>GMFLLQGAQMLQMLEKSLRKSLPMSLKVYGTVMHMNHGNPFNLKALVDKWPDFQTVVIRPQEQDMKDDLDHYTNTYHVYSEDLKNCQEFLDLPEVINWKQHLQIQSTQSSLNEVIQNLAATKSFKVKRSKNILYMASETIKE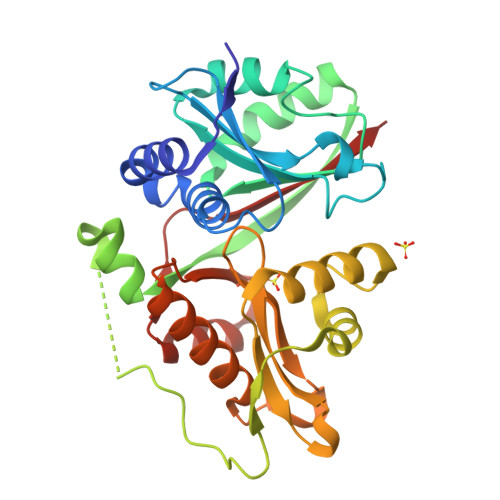LTPSLLDVKNLPVGDGKPKAIDPEMFKLSSVDPSHAAVVNRFWLFGGNERSLRFIERCIQSFPNFCLLGPEGTPVSWSLMDQTGEMRMAGTLPEYRAQGLVTHAIYQQAQCLLKRGFPVYSHVDPKNQIMQKMSQSLNHVPMPSDWNQWNCEPL[2x]> GSGHKSSPCDTNWRYYGDSCYGFFRHNLTWEESKQYCTDMNATLLKIDNRNIVEYIKARTHLIRWVGLSRQKSNEVWKWEDGSVISENMFEFLEDGKGNMNCAYFHNGK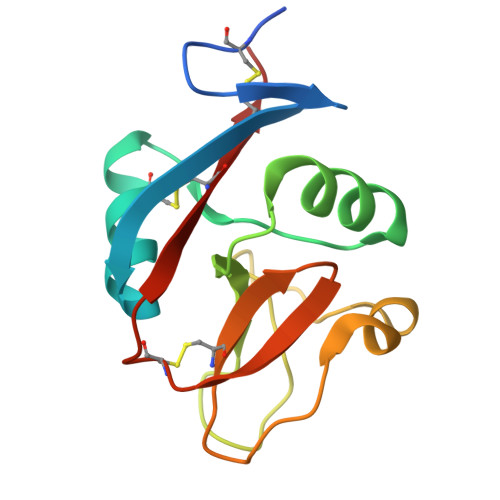MHPTFCENKHYLMCERKAG>[2x]MLSPIRTTFHNSVNIVQSSPSQTVSFAGKEYELKVIDEKTPILFQWFEPNPERYKKDEVPIVNTKQHPYLDNVTNAARIESDRMIGIFVDGDFSVNQKTAFSKLERDFENVMIIYREDVDFSMYDRKLSDIYHDIICEQRLRTEDKRDEYLLNLLEKELREISKAQDSLISMYAKKRNHAWFDFFRNLALLKAGEIFRSTYNTKNHGISFGEGCIYLDMDMILTGKLGTIYAPDGISMHVDRRNDSVNIENSAIIVNRSNHPALLEGLSFMHSKVDAHPYYDGLGKGVKKYFNFTPLHNYNHFCDFIEFNHPNIIMNTSQYTCSSW

The non-LEE encoded effector protein B (NleB) has GT activity and inhibits NF-κB activation by transferring N-acetyl glucosamine (GlcNAc) to host death domain-containing proteins and to glyceraldehyde 3-phosphate dehydrogenase (GAPDH). The glycosylation target is an arginine residue, which was unexpected because the guanidine group of arginine is nucleophilically poor at physiological pH. The T3SS effectors SseK1 and SseK2 from Salmonella typhimurium SL1344 are NleB orthologs that behave as NleB1-like GTs, although they differ in protein substrate specificity. Here, by using a combination of X-ray crystallography, STD-NMR, enzyme kinetics, molecular dynamics simulations, and in vivo experiments, we show that these enzymes are GT-A fold retaining GTs that most likely follow an SNi mechanism.

NleB2 from E. coli O145:H28 was solved in its unliganded form. For NleB2, amino acids 317–326 at the C-terminus were deleted for better crystal packing and Cys21 and Cys199 were also substituted to serine. The overall crystal structures of SseK1 and SseK2 from S. typhimurium as well as NleB2 from enteropathogenic E. coli are similar, revealing high identities between the amino acids at the active binding site level. Furthermore, the sequence alignment shows that the NleB family lacks the arginine residue, though a conserved Trp is present at the C-terminus. We would expect that both the SseK and NleB families have a different conformational behavior of the lid-domain. Each HEN residue of SseK3 is on the β-strand, but in the case of SseK1, SseK2, and NleB2, the HEN residues are located on the loop structure. This has implications for the differences in the activity of the enzymes due to the HEN motif because the loop structure is more flexible than the β-strand. Although the tertiary structure of NleB1 is likely similar to NleB2, SseK1, and SseK2, a previous study has reported that NleB2 has a lower activity than NleB1 on the same target (TRADD).>[4x]S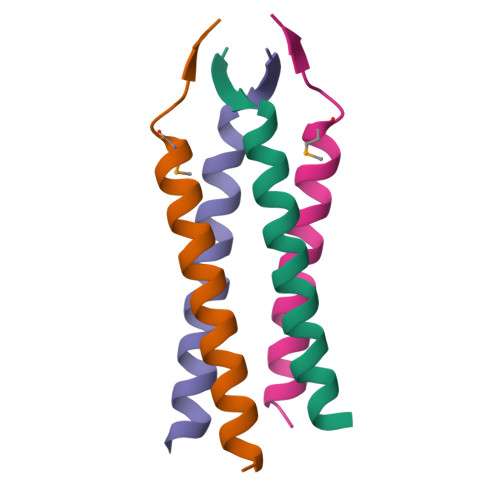YYIDADLLREIKQHLKQQQEGLSHLISIIKDDMEDIKLV>[2x]HMVPMDKTLKEFGADVQWDDYAQLFTLIKDGAYVKVKPGAQTAIVNGQPLALQVPVVMKDNKAWVSDTFINDVFQSGLDQTFQVEKRPHPLNALTADEIKQAVEIVKASADFKPNTRFTEISLLPPDKEAVWAFALENKPVDQPRKADVIMLDGKHIIEAVVDLQNNKLLSWQPIKDAHGMVLLDDFASVQNIINNSEEFAAAVKKRGITDAKKVITTPLTVGYFDGKDGLKQDARLLKVISYLDVGDGNYWAHPIENLVAVVDLEQKKIVKIEEGPVVPVPMTARPFDGRDRVAPAVKPMQIIEPEGKNYTITGDMIHWRNWDFHLSMNSRVGPMISTVTYNDNGTKRKVMYEGSLGGMIVPYGDPDIGWYFKAYLASGDYGMGTLTSPIARGKDAPSNAVLLNETIADYTGVPMEIPRAIAVFERYAGPEYKHQEMGQPNVSTERRELVVRWISTVGN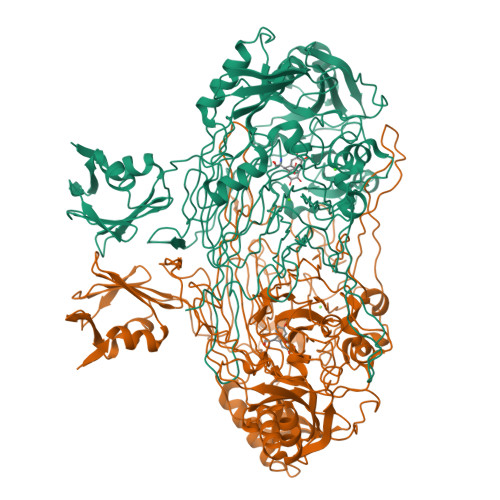YDYIFDWIFHENGTIGIDAGATGIEAVKGVKAKTMHDETAKDDTRYGTLIDHNIVGTTHQHIYNFRLDLDVDGENNSLVAMDPVVKPNTAGGPRTSTMQVNQYNIGNEQDAAQKFDPGTIRLLSNPNKENRMGNPVSYQIIPYAGGTHPVAKGAQFAPDEWIYHRLSFMDKQLWVTRYHPGERFPEGKYPNRSTHDTGLGQYSKDNESLDNTDAVVWMTTGTTHVARAEEWPIMPTEWVHTLLKPWNFFDETPTLGALKKDK> MHHHHHHMTRQEIFQEQLAAVPEFRGLGPLFKSSPEPVALTESETEYVIRCTKHTFTNHMVFQFDCTNTLNDQTLENVTVQMEPTEAYEVLCYVPARSLPYNQPGTCYTLVALPKEDPTAVACTFSCMMKFTVKDCDPTTGETDDEGYEDEYVLEDLEVTVADHIQKVMKLNFEAAWDEVGDEFEKEETF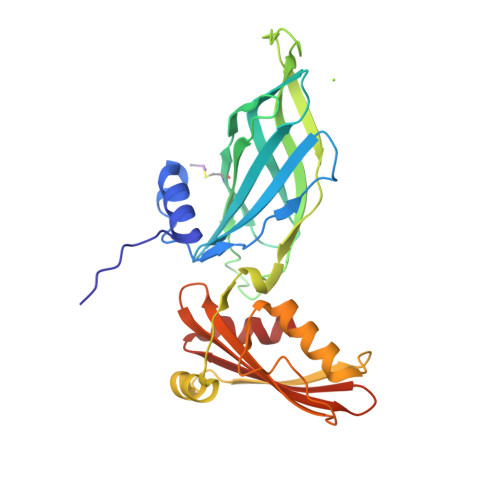TLSTIKTLEEAVGNIVKFLGMHPCERSDKVPDNKNTHTLLLAGVFRGGHDILVRSRLLLLDTVTMQVTARSLEELPVDIILASVG> MGSSHHHHHHSSGLVPRGSHSDEVDAHMESNDSGGVAAKHGFLFQDCVAAYHVTRMLRDKTIRSVRCEVTDDIDIVSDGYIDFVQVKSTGKTRWNISDIVQNSKGADKKTIPCSSILHKSMQCESDLSLGRRYSIVTEEKVNKTLEYLTISPNARLDKPGRQELIDDLNKRTDNFLTDSGISVSDWIDAATWEVFSSLRELELLGIKNIRLASQDLHGVILSSETVAEDIWCRILDTVTRKGEHSRRIHSADDKSYLRPDLLEWFKQRVEDDQSRSGRKIYVKRDLPHILTPFRAPMASVCAKRKGQVLHQQYSLKKYRYKHIADNVCQWLDEVFLRPKEMSDIHKLTFIEKRERLKNSVFKSLHDVSEFLGRVLLHATIRQHHESQPIPCMLYVEKAGAEKILENVHIVRRDPEGDQLWIGFSELVTDINIAVRLPEIRDQLYEDISDCIDTARKKILDIKDDNYLLRHDIDEILDGSQPFDAHLDRFTFVLFVGYDSNLLTEPETPGFEDDLEKETAVLFEKFAADLIEDSPFANLCIHVFIYPAPSLERLTQLVDEKVREVV;> MTEIYEQAKHSLQGEDFSSFNYLFAVNKLLSNPVSY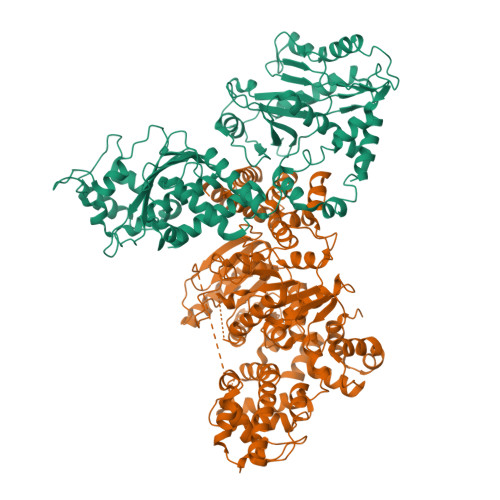DLGRDLIVRALDSRERFSEHTTILKNMVRKSGLFPYLKKEFTSLTPDDLRVLELYRTPFSDGYVFHSMQFHIFDLLKSGQNVVLSAPTSMGKSAIVDSLLGMGTLKRLVLVVPTVALADETRRRLQERFGDRYQIIHHSSQVCHSDQAVYVLTQERVNERDDIVDIDLFVIDEFYKLAFRQLKSGDIDHQDERVIELNIALSKLLKVSRQFYLTGPFVNSIRGLEKLGYPHTFVSTDFNTVALDVKTFGIKANDDKAKLKALGEIAHACVDATIIYCKSPTVAGLVARELIRLGHGTPTENPHVDWVSEEFDADWDYTVALRNGIGLHFGALPRALQQYTADQFNAGKLRFLLCTSTIIEGVNTIAKNVVIYDNRDGTRSIDKFTHGNIKGRAGRMGVHFVGKIFCLEEIPEDNLNQEVDIPLGIQGIDTPINLLASVQPDHLSEFSQDRFDEVFINDRVSIDLVKKHSYFRVEQFEMLQSMFEMMDDNEFSSLVFHWTPATNFLKTFAKIIARLVPHTFSRNGVPVKPTDVMIAKLAGYLSAESYSEYLKNQIDYARQWISEGEKRTLSIALNNDLKLITNTFGYTLPKVLSLMEDVVKHHAVKRGIRSKVDYTHVKLAFESFHLPPGVNALEEIGIPIQTLHRLVDLLEFSDEADVDELSQYLRDTQDIWSRSIGYVDQMFIRRALGIRRH Erythromycin B | C37 H67 N O12 | 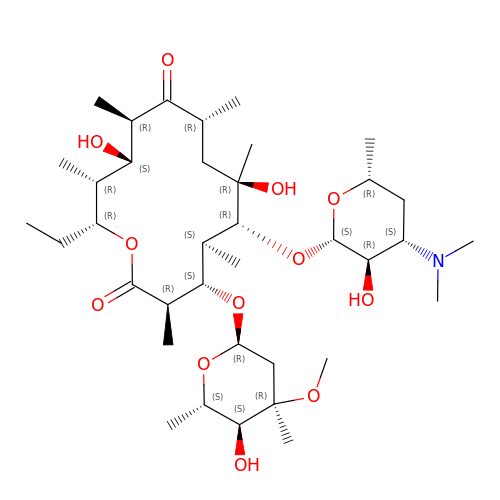IDRYSCOQVVUBIJ-PPGFLMPOSA-N> MSGIPEITAYPLPTAQQLPANLARWSLEPRRAVLLVHAMQRYFLRPLPESLRAGLVANAARLRRWCVEQGVQIAYTAQPGSMTEEQRGLLKDFWGPGMRASPADREVVEELAPGPDDWLLTKWRYSAFFHSDLLQRMRAAGRDQLVLCGVYA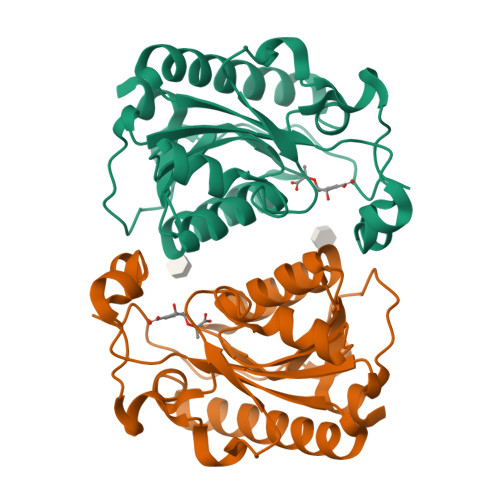HVGVLISTVDAYSNDIQPFLVADAIADFSEAHHRMALEYAASRCAMVVTTDEVLE>DALGTGNAQKQQDINHLLDKIYEPTKYPDLKDIAENFNPLGDTSIYNDHGAAVETLMKELNDHRLLEQRHWYSLFNTRQRKEALMLFAVLNQCKEWYCFRSNAAYFRERMNEGEFVYALYVSVIHSKLGDGIVLPPLYQITPHMFTNSEVIDKAYSAKMTQKPGTFNVSFTGTKKNREQRVAYFGEDIGMNIHHVTWHMDFPFWWEDSYGYHLDRKGELFFWVHHQLTARFDFERLSNWLDPVDELHWDRIIREGFAPLTSYKYGGEFPVRPDNIHFEDVDGVAHVHDLEITESRIHEAIDHGYITDSDGHTIDIRQPKGIELLGDIIESSKYSSNVQYYGSLHNTAHVMLGRQGDPHGKFNLPPGVMEHFETATRDPSFFRLHKYMDNIFKKHTDSFPPYTHDNLEFSGMVVNGVAIDGELITFFDEFQYSLINAVDSGENIEDVEINARVHRLNHNEFTYKITMSNNNDGERLATFRIFLCPIEDNNGITLTLDEARWFCIELDKFFQKVPSGPETIERSSKDSSVTVPDMPSFQSLKEQADNAVNGGHDLDLSAYERSCGIPDRMLLPKSKPEGMEFNLYVAVTDGDKDTEGHNGGHDYGGTHAQCGVHGEAYPDNRPLGYPLERRIPDERVIDG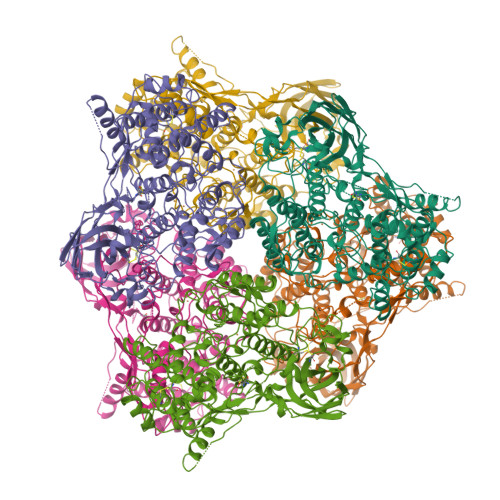VSNIKHVVVKIVHHLEHHD[6x]Members of the Vaccinia-related kinase (VRK) family of serine/threonine protein kinases are present in the genomes of all metazoans and those of poxviruses, including the family-founding member vaccinia virus B1R1–6. Here we present the first crystal structures of the kinase domain of VRK1 and the first crystal structures for ligand-bound VRK1 and VRK2. Ligand-bound VRK kinase domains adopt the canonical protein kinase fold, except for the presence of the additional α-helix between αC and β4 (αC4) exclusively found on VRK proteins. The ligand-bound structures obtained here for active VRKs are in a closed, active conformation and display the same overall organization previously observed for the apo-structures, including the position of the VRK-exclusive αC4 and the structural organization of conserved residues that make up the kinase hydrophobic spine36.

For both VRK13-364 and VRK214-335, the compound inducing the largest ΔTm shift was BI-D1870, a dihydropteridinone inhibitor originally developed for p90 RSK (ribosomal S6 kinase)32 which displayed more substantial temperature stabilization than the best PKIS hit for VRK13-364, GW297361X (5.5 versus 3.9 °C in this experiment, respectively). Nevertheless, the most complete polypeptide chain in this model contains an intact P-loop (chain A, residues 22–341; used for the structural comparisons below). The VRK214-335/BI-D1870 model contains residues 14–328 and also has a complete P-loop. BI-D1870 adopts a non-planar conformation that complements well the ATP-binding site of VRK2. However, the VRK2/BI-D1870 co-structure revealed this protein favors a particular enantiomer of BI-D1870 (S-form) and that the methyl group attached to the stereogenic center projects into a cavity formed by the hydrophobic side chains from P-loop residues. The pendant isopentyl group in the bicyclic core is orthogonal to the plane of the ring in a configuration that allows Gly39 from the P-loop to approach Asp186 in the DYG motif, closing the P-loop over the compound 3,5-difluoro-4-hydroxyphenyl ring. Structural comparisons of ligand-bound and apo-VRK2 structures reveal the isopentyl moiety also orients the side chain of Asp186 towards the catalytic lysine. For example, the gatekeeper methionine is displaced and the catalytic lysine re-positions itself to become the focal point in a network of polar contacts that also involves the phenol of BI-D1870 and the side chains of Asp186 and that from the conserved glutamate residue in αC, Glu73. By contrast, in VRK214-335, both main chain and side chain atoms in the P-loop are in close proximity to atoms from the compound. Thus, the folded conformation of the P-loop in VRK2 seems to be driven mostly by shape complementarity and hydrophobic contacts between the protein and the compound, whereas in VRK1 the P-loop folded conformation is held in place by a direct interaction between the ligand sulfur atom and the protein aromatic residue.

> SMPFPEGKVLDDMEGNQWVLGKKIGSGGFGLIYLAFPTNKPEKDARHVVKVEYQENGPLFSELKFYQRVAKKDCIKKWIERKQLDYLGIPLFYGSGLTEFKGRSYRFMVMERLGIDLQKISGQNGTFKKSTVLQLGIRMLDVLEYIHENEYVHGDIKAANLLLGYKNPDQVYLADYGLSYRYCPNGNHKQYQENPRKGHNGTIEFTSLDAHKGVALSRRSDVEILGYCMLRWLCGKLPWEQNLKDPVAVQTAKTNLLDELPQSVLKWAPSGSSCCEIAQFLVCAHSLAYDEKPNYQALKKILNPHGIPLGPLDFSTKGQSINVH> GHMAKKKATETTDEDEDGGSEKKYRKCEKAGCTATCPVCFASASERCAKNGYTSRWYHLSCGEHFCNECFDHYYRSHKDGYDKYTTWKKIWTSNGKTEPSPKAFMADQQLPYWVQCTKPECRKWRQLTKEIQLTPQIAKTYRCGMKPNTAIKPETSDHCSLPEDLRVLEVSNHWWYSMLILPPLLKDSVAAPLLSAYYPDCVGMSPSCTSTNRAAATGNASPGK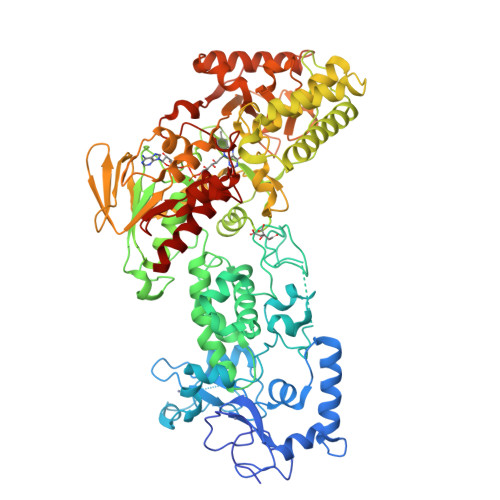LEHSKAALSVHVPGMNRYFQPFYQPNECGKALCVRPDVMELDELYEFPEYSRDPTMYLALRNLILALWYTNCKEALTPQKCIPHIIVRGLVRIRCVQEVERILYFMTRKGLINTGVLSVGADQYLLPKDYHNKSVIIIGAGPAGLAAARQLHNFGIKVTVLEAKDRIGGRVWDDKSFKGVTVGRGAQIVNGCINNPVALMCEQLGISMHKFGERCDLIQEGGRITDPTIDKRMDFHFNALLDVVSEWRKDKTQLQDVPLGEKIEEIYKAFIKESGIQFSELEGQVLQFHLSNLEYACGSNLHQVSARSWDHNEFFAQFAGDHTLLTPGYSVIIEKLAEGLDIQLKSPVQCIDYSGDEVQVTTTDGTGYSAQKVLVTVPLALLQKGAIQFNPPLSEKKMKAINSLGAGIIEKIALQFPYRFWDSKVQGADFFGHVPPSASKRGLFAVFYDMDPQKKHSVLMSVIAGEAVASVRTLDDKQVLQQCMATLRELFKEQEVPDPTKYFVTRWSTDPWIQMAYSFVKTGGSGEAYDIIAEDIQGTVFFAGEATNRHFPQTVTGAYLSGVREASKIAAF>[3x]MFSKFFIERPVFASVVAIIISLAGAIGLTNLPIEQYPSLTPPTVKVSATYTGADAQTIASTVASPIEDAINGADNMIYMDSTSSSSGTMSLTVYFDIGTDPDQATIDVNNRISAATAKMPDAVKKLGVTVRKTSSTTLAAISMYSSDGSMSAVDVYNYITLNVLDELKRVPGVGDANAIGNRNYSLRIWLKPDLLNKFGITATDVISAVNDQNAQYATGKIGEEPVTQKSPYVYSITMQGRLQNPSEFENIILRTNNDGSFLRLKDVADVEIGSQQYSSQGRLNGNDAVPIMINLQSGANALHTAELVQAKMQELSKNFPKGLTYKIPYDTTKFVIESIKEVVKTFVEALILVIIVMYMFLKNFRATLIPMIAVPVSLLGTFAGLYVLGFSINLLTLFALILAIGIVVDDAIIVVENIDRILHENEQISVKDAAIQAMQEVSSPVISIVLVLCAVFVPVSFISGFVGEIQRQFALTLAISVTISGFVALTLTPSLCALFLRRNEGEPFKFVKKFNDFFDWSTSVFSAGVAYILKRTIRFVLIFCIMLGAIFYLYKAVPNSLVPEEDQGLMISIINLPSASALHRTISEVDHISQEVLKTNGVKDAMAMIGFDLFTSSLKENAAAMFIGLQDWKDRNVSADQIIAELNKKFAFDRNASSVFIGLPPIPGLSITGGFEMYVQNKSGKSYDEIQKDVNKLVAAANQRKELSRVRTTLDTTFPQYKLIIDRDKLKHYNLNMQDVFNTMNATIGTYYVNDFSMLGKNFQVNIRAKGDFRNTQDALKNIFVRSNDGKMIPLDSFLTLQRSSGPDDVKRFNLFPAAQVQGQPAPGYTSGQAIEAIAQVAKETLGDDYSIAWSGSAYQEVSSKGTASYAFALGMIFVFLILAAQYERWLIPLAVVTAVPFAVFGSFLLVYLRGFSNDIYFQTGLLLLIGLSAKNAILIVEFAMEERFKKGKGVFEAAVAAAKLRFRPIIMTSLAFTFGVLPMIFATGAGSASRHSLGTGLIGGMIAASTLAIFFVPLFFYLLENFNEWLDKKRGKVHE

The Cme locus consists of three tandemly linked genes (cmeABC) encoding protein components of the tripartite Cme efflux pump (CmeA, CmeB, and CmeC), where all three components are absolutely required for substrate expulsion. This tripartite system is composed of the CmeB efflux pump, an inner membrane resistance-nodulation-cell division (RND)12 transport protein that contains substrate-binding sites and transduces the electrochemical energy required for pumping drugs out of the cell; the CmeA periplasmic protein, a member of the membrane fusion protein family; and the CmeC outer membrane-associated protein that is integral to the outer membrane. To understand the transport mechanism of the CmeB efflux pump from C. jejuni, we here define the X-ray structures of this membrane protein, which assembles as a trimer. Overall, CmeB adopts the fold of a typical hydrophobe-amphiphile efflux (HAE)-RND-type protein and forms a homotrimer, with its pseudo threefold symmetrical axis positioning perpendicular to the membrane surface. Each subunit of CmeB contains 12 transmembrane helices (TM1-TM12) and a large periplasmic domain created by two extracellular loops between TM1 and TM2, and between TM7 and TM8, respectively.

Two distinct conformations of CmeB with space groups C2 (form I) and P1 (form II) were captured in two different forms of crystals. In the form I structure, the three periplasmic clefts of the CmeB trimer are closed. Although the conformations of the three monomers are different from each other, they are more similar to the “extrusion” form of AcrB. A channel for extrusion is found in each protomer of our form I structure. We therefore assigned the conformational state of these three protomers as the “extrusion” form. All of the extrusion protomers in both form I and form II crystals share very similar structural features, which include the conformation of transmembrane helices and position of side chains of residues within the proton-relay network such as D409 and D410 of TM4 and K935 of TM10. For the asymmetric CmeB trimer, the conformations of the three protomers display in such a way that either only one out of the three periplasmic clefts is open or all of these clefts are closed.> SVDHGFLVTRHSQTTDDPQCPPGTKILYHGYSLLYVQGNERAHGQDLGTAGSCLRKFSTMPFLFCNINNVCNFASRNDYSYWLSTPEPMPMSMAPITGENIRPFISRCAVCEAPAMVMAVHSQTIQIPQCPTGWSSLWI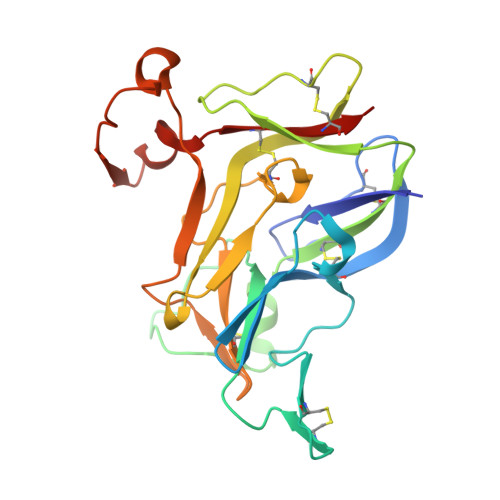GYSFVMHTSAGAEGSGQALASPGSCLEEFRSAPFIECHGRGTCNYYANAYSFWLATIERSEMFKKPTPSTLKAGELRTHVSRCQVCMRRT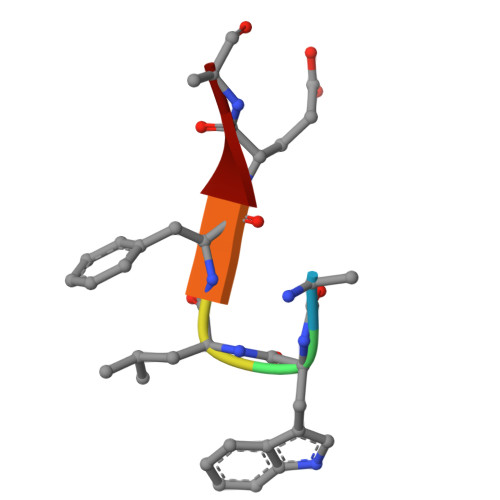> AWLFEA>[2x]MDFTKEKFQLLAISSLTLPWLISLAFNYHHPALTQTLLSGLAVVSASFLISWAAETAEMDVPRSFSLAIVALLAVLPEYAVDGYFAWKAGSVGGEYVHYATANMTGANRLLIGIGWSLVAFIAFRTLKSKEVELDDGIRLEIFFLFLATLYAFTLPLKGHISPFDALVFVSLYAIYIYLSTKAEREEVEVGGVPAYLCSLKTETRRLS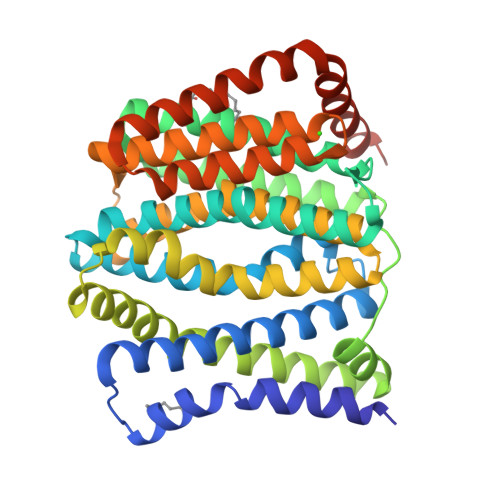VVVLFLFAGFTILMSVEAFSEGLLETARIAGIDEFLAVQWIAPLASESPELIVAIYFVRRFRVSASMNALISSKVNQWTLLIGTIAIIYSISAFKLQSLPLDARQSEEVLLTAAQSLFAVAILLDLKISWKEASALFLLFIVQLLFPGVEVRYIISAIYIILSLPILFAKRKEIVESFRTVKRLISLESSGENLYFQ>MSQHNEKNPHQHQSPLHDSSEAKPGMDSLAPEDGSHRPAAEPTPPGAQPTAPGSLKAPDTRNEKLNSLEDVRKGSENYALTTNQGVRIADDQNSLRAGSRGPTLLEDFILREKITHFDHERIPERIVHARGSAAHGYFQPYKSLSDITKADFLSDPNKITPVFVRFSTVQGGAGSADTVRDIRGFATKFYTEEGIFDLVGNNTPIFFIQDAHKFPDFVHAVKPEPHWAIPQGQSAHDTFWDYVSLQPETLHNVMWAMSDRGIPRSYRTMEGFGIHTFRLINAEGKATFVRFHWKPLAGKASLVWDEAQKLTGRDPDFHRRELWEAIEAGDFPEYELGFQLIPEEDEFKFDFDLLDPTKLIPEELVPVQRVGKMVLNRNPDNFFAENEQAAFHPGHIVPGLDFTNDPLLQGRLYSYTDTQISRLGGPNFHEIPINRPTCPYHNFQRDGMHRMGIDTNPANYEPNSINDNWPRETPPGPKRGGFESYQERVEGNKVRERSPSFGEYYSHPRLFWLSQTPFEQRHIVDGFSFELSKVVRPYIRERVVDQLAHIDLTLAQAVAKNLGIELTDDQLNITPPPDVNGLKKDPSLSLYAIPDGDVKGRVVAILLNDEVRSADLLAILKALKAKGVHAKLLYSRMGEVTADDGTVLPIAATFAGAPSLTVD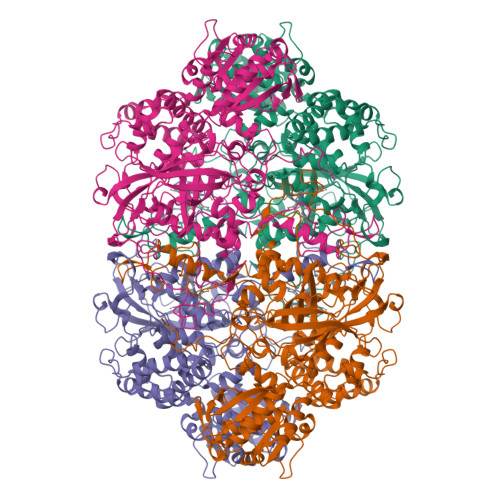AVIVPCGNIADIADNGDANYYLMEAYKHLKPIALAGDARKFKATIKIADQGEEGIVEADSADGSFMDELLTLMAAHRVWSRIPKIDKIPA[4x]>[4x]TITLTENKRKSMEKLSVDGVISALAFDQRGALKRMMAQHQTKEPTVEQ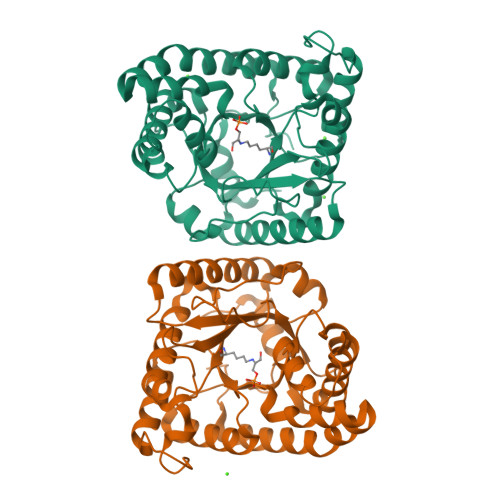IEELKSLVSEELTPFASSILLDPEYGLPASRVRSEEAGLLLAYEKTGYDATTTSRLPDCLDVWSAKRIKEAGAEAVKFLLYYDIDGDQDVNEQKKAYIERIGSECRAEDIPFYLEILTYDEKIADNASPEFAKVKAHKVNEAMKVFSKERFGVDVLKVEVPVNMKFVEGFADGEVLFTKEEAAQAFRDQEASTDLPYIYLSAGVSAKLFQDTLVFAAESGAKFNGVLCGRATWAGSVKVYIEEGPQAAREWLRTEGFKNIDELNKVLDKTASPWTEKM> GAMGSTAEQKTKAKVLLEEGSFLGYEDKLRQRLKLGKDDRPSVSLWSVLKSMVGKDMTRMTLPVSFNEPTSLLQRVAEDLEYADLLNQAASFEDSTLRLLYVAIFTVSSYASTVKRVAKPFNPLLGETFEYSRPDKSYRFFTEQVSHHPPISATWTESPKWDFFGESFVDSKFNGRSFDFKHLGLWYLTIRPDSNGKEELYTYKKPNNQVVGILLGNPQVDNYGDVKIVNHNTGDYCMIHFKARGWRSSSAYEVKGEVYNAKGGKEWIFGGRWNESVSAKKVLKPNSLEEMQVDELKHSVTHTSSGGPKYDGTRFNVWHVNERPEFPFNLTKFAV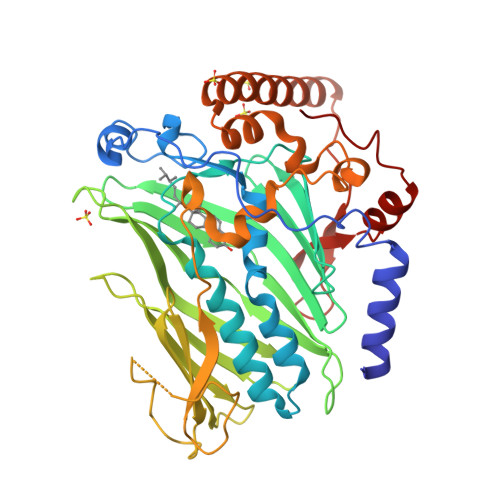TLNAPQPHLLPWLPPTDTRLRPDQRAMEEGRYDEAATEKHRVEERQRSVRKKREEKNITYQQRWFKKEIHPVTKCDYWKFNGEYWKQRRDHKLADEGDIF>MFYQPAQNKKQYDDLADIEAQNNVPNTQEVLEAWQESLDSDEDESSPLEESNGFTISEHDDFVKSVPRKNNPTDLLYSGKLLDSDEPPSVHGNSSKVPSKHPSPSFPETTSLRNLQNGSKQKPALPNFNDPHFYNEDVTRSGHPNRSIYTQLPRNEFSNARVLWNRLSARDRVLWRWANVENLDSFLQQVYTYYTGKGLSCIIVHRLFQILTVSFVIGFTTFITSCIDWPAVTPHGSLAGVTKSQCIAQMSPITYLVLWLFLSFLLALWIYYLTDIPRLWQMREFYIHALKIATADMPTVSWQRVLYRLLKLKNVNALTAEDGRVVSLHNMKRLDAYAIANRIMRKDNYFIALINNGIINIELPLLHRRILTHTTEWNINWCIFNFVFDEQGQLRSAFRNPNSRKRLSEELRRRFIVAGFLNCLFAPIVAIYLVIHNFFRYFNEYHKNPGALSTRRYTPLALWTFREYNELQHFFDERINDSYAAASHYVSQFPDFNMIRLFKYISFILGSFTAILVIITVFDPELMVTFEITKDRSVLFYLGLFGSLIAVSRSIIPDETLVFAPEKALRRVITFTHYMPGWWSDNMHSKAVQQEFCSLYSYRIVNLLWEILGILLTPVLLFFTFPSCSQDIVDFFREHTINVEGVGYVCSYAVFQDNPPYESVASLVQSRKISPLIQNKP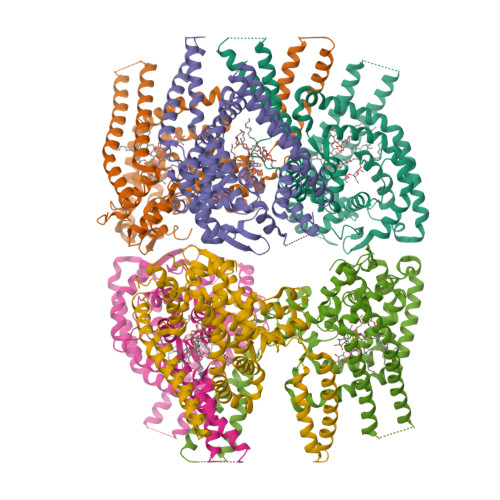ELSRIYFYEQFNTEAPRRDLRGSLEVLFQ[6x]> MGSSHHHHHHSQDPKRPMDTEEAEELVRQWENVKAEALGPTHQVYSLSEVLDESMLVQWQTLAQTAEAKSCYWRFV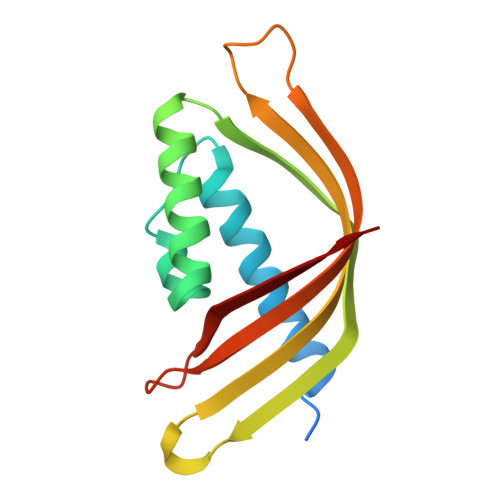LLHLEVLQAHIFEDGIAGEAAEIEALLEEAAELVDESQPKNAKYYSTYKIRYILKKQEDGLWKFCQSDIQIQK Anti-chemokine activity has been described in the extracts of tick salivary glands, and we have recently described the cloning and characterization of such chemokine binding proteins from a tick salivary gland cDNA library, which we have named Evasins. Evasin-1 is a small 94-amino acid protein which binds CCL3/MIP-1α and CCL4/MIP-1β with very high affinity (0.16 and 0.81 nM, respectively), and also displays lower affinity binding (3.2 nM) to a closely related member of the CC chemokine family, CCL18/ PARC. This chemokine-binding protein does not share any relevant sequence or structural homology to any other known proteins, notably the viral chemokine-binding proteins, and moreover, is considerably smaller, being only 10 kDa compared to the viral proteins which range in size between 30–40 kDa. The Evasin-1 secondary structure is composed of seven beta strands forming three anti-parallel beta sheets, one short alpha helix, and contains four disulfide bridges.

We have determined the crystal structure of both non-glycosylated (accession code: 3 fpr) and glycosylated Evasin-1 (accession code: 3 fpt), to 1.7 Å and 2.70 Å respectively. In order to obtain non-glycosylated protein, Evasin-1 was expressed in the presence of tunicamycin, a known inhibitor of N-linked glycosylation. The crystal structure of the non-glycosylated Evasin-1 contains two molecules per asymmetric unit, monomer A (Asp5-Asp91) and monomer B (Gly10-Trp89). In both monomers, the extreme N-terminal and C-terminal regions, comprising the six-histidine tag, are flexible and were not seen in the electron density maps. The overall structure of the Evasin-1 molecule is boat shaped, with approximate dimensions of 35 Å × 20 Å × 13 Å. The four disulfide bridges consist of: Cys12-Cys33 connecting the N-terminal region of strand β1with β3; Cys29-Cys70 connecting the beginning of β3 with β6; Cys46-Cys75 connecting the strands β5 with β7 in the beta sheet β5-β6-β7 and finally Cys65-Cys84 connecting the other two strands β6 with β7 in the same beta sheet. The disulfide bridges are positioned along the interior of the protein, forming a central core, and undoubtedly conferring structural rigidity by stabilization of the protein core. The N-terminal region is anchored not only by the disulfide bridge, but also by an intricate hydrogen bond network that places the N-terminal segment in an exposed and favourable position for chemokine binding. The C-terminal loop points to the solvent, presenting the aromatic residue Trp89 totally exposed and located in a flexible region with a Cα B-factor = 50.0 Å2, much higher than the average B-factor  = 34.8 Å2 for the whole protein chain of monomer A (B-factor for the Cα of monomer A  = 32.8 Å2, calculated with BAVERAGE from CCP4, 1994).

>EDDEDYGDLGGCPFLVAENKTGYPTIVACKQDCNGTTETAPNGTRCFSIGDEGLRRMTANLPYDCPLGQCSNGDCIPKETYEVCYRRNWRDKKNHHHHHH[2x]>VLTGLEPVRRRPGMYTDTTRPNHLGQEVIDNSVDEALAGHAKRVDVILHADQSLEVIDDGRGMPVDIHPEEGVPAVELILCRLHAGGKFSNKNYQFSGGLHGVGISVVNALSKRVEVNVRRDGQVYNIAFENGEKVQDLQVVGTCGKRNTGTSVHFWPDETFFDSP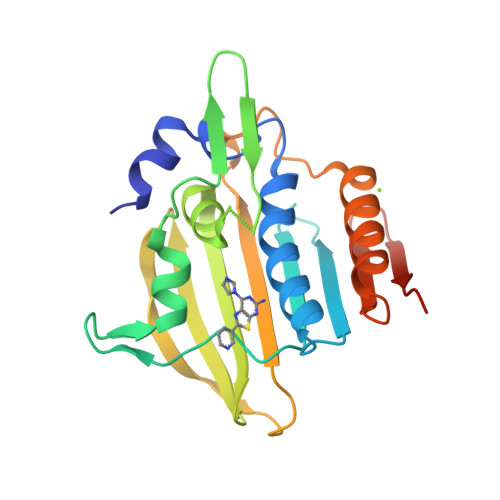RFSVSRLTHVLKAKAVLCPGVEITFKDEINNTEQRWCYQLEHHHHHH[2x]>MREKLFWILKKYGVSDHIAKAFLEIPREEFLTKSYPLSYVYEDIVLVSYDDGEEYSTSSQPSLMALFMEWVGLDKGMRVLEIGGGTGYNAAVMSRVVGEKGLVVSVEYSRKICEIAKRNVERLGIENVIFVCGDGYYGVPEFSPYDVIFVTVGVDEVPETWFTQLKEGGRVIVPINLKLSRRQPAFLFKKKDPYLVGNYKLETRFITAGGNLGNLLERNRKLLREFPFNREILLVRSHIFVELVDLLTRRLTEIDGTFYYAGPNGVVEFLDDRMRIYGDAPEIENLLTQWESCGY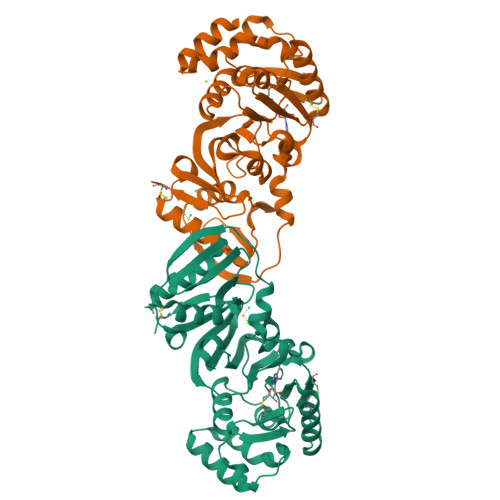RSFEYLMLHVGYNAFSHISCSI[2x]>MHHHHHHSSGRENLYFQGRKTLVLIGASGVGRSHIKNALLSQNPEKFVYPVPYTTRPPRKSEEDGKEYHFISTEEMTRNISANEFLEFGSYQGNMFGTKFETVHQIHKQNKIAILDIEPQTLKIVRTAELSPFIVFIAPTDQ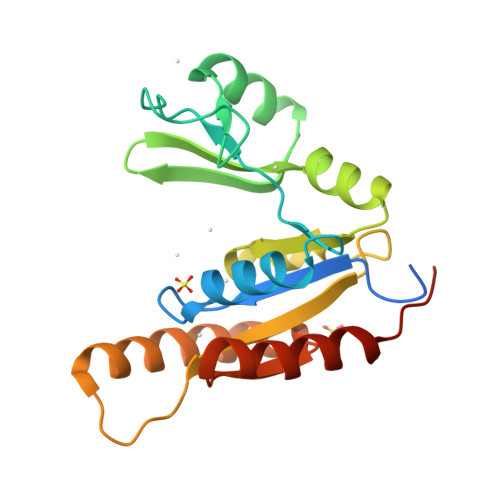GTQTEALQQLQKDSEAIRSQYAHYFDLSLVNNGVDETLKKLQEAFDQACSSPQWV[6x]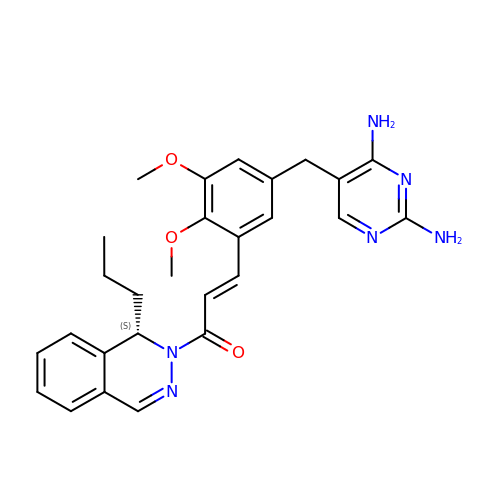5-(3,4-dimethoxy-5-{(1E)-3-oxo-3-[(1S)-1-propylphthalazin-2(1H)-yl]prop-1-en-1-yl}benzyl)pyrimidine-2,4-diamine | C27 H30 N6 O3 | YGDVMSPWZQHNMB-NEQMZLFVSA-N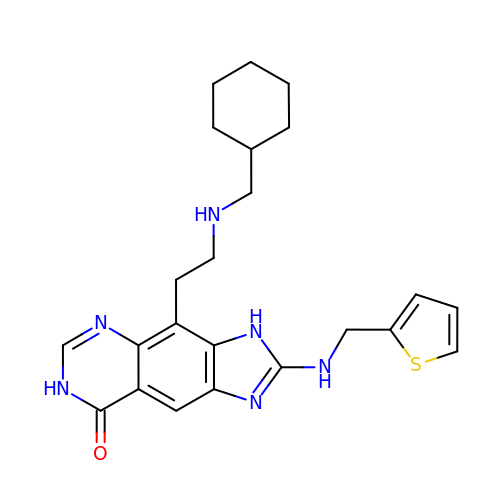4-{2-[(cyclohexylmethyl)amino]ethyl}-2-[(thiophen-2-ylmethyl)amino]-3,7-dihydro-8H-imidazo[4,5-g]quinazolin-8-one | C23 H28 N6 O S | YNWRNLSOYRMCNY-UHFFFAOYSA-N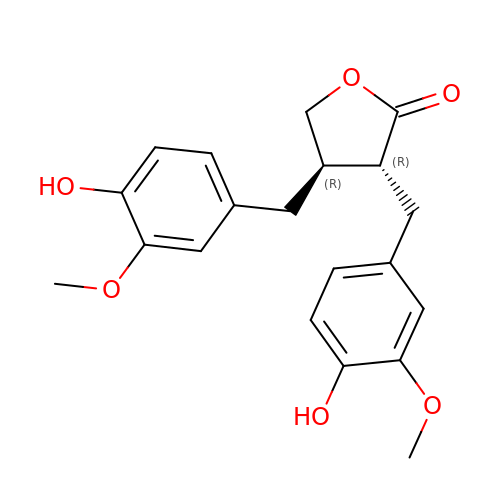MATAIRESINOL | C20 H22 O6 | MATGKVZWFZHCLI-LSDHHAIUSA-N3-[(E)-{4-formyl-5-hydroxy-6-methyl-3-[(phosphonooxy)methyl]pyridin-2-yl}diazenyl]-7-nitronaphthalene-1,5-disulfonic acid | C18 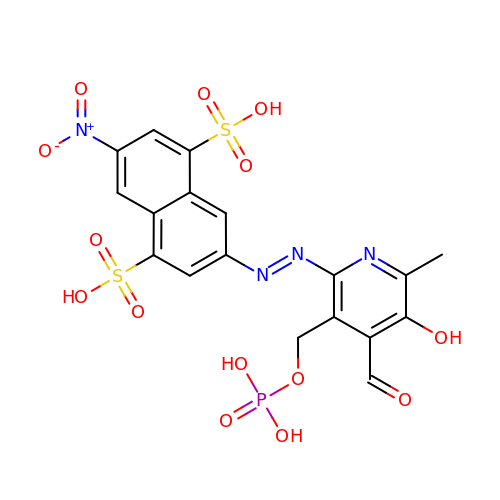H15 N4 O14 P S2 | CMVLDSZYDWJTCG-QZQOTICOSA-N>[2x]MQRLGTAVFFLLAFRYSTEQAVGLKEPNAPCTTACGCKSRLLKRLDLYTSKYADGINNERENSEAYSKLVTAALAAVPTMQRKILPLLGAAADILDICRRELATARPLVQAAISKIEEAAGVYNTLHKLERGLG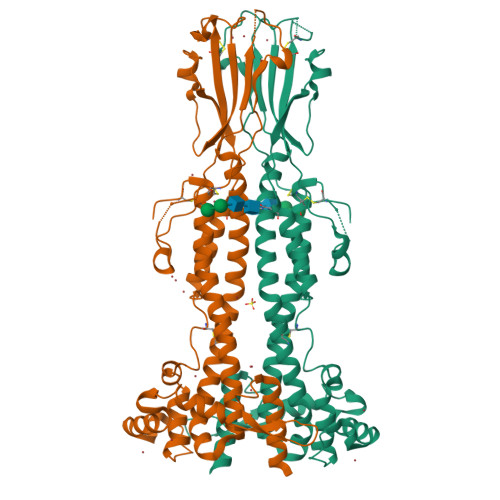EAKIEFGGTDLRLTKTKFRATSLGTIHTADCPNADPGETNVKIGLEHEENEPEPAKLITHGHLDATCASGVGQSSSCHTTAVEANTHLTLGLTFSGSSKDESATWNAATNNKRAIHSNDADFLGSNATVAHEALKAIRSAGASTPCSSLITDFNAVRANPKFKLMVIKALLNKPTAEKESDAPADEVNNAINSAYGREGSEYNTKTWKDIGSTRIPKADPPGEKTDTIDKLSSLPQWGDAIARLLLQEITKQEEQSIKTSSDEATNKECDKHTAKTEGECTKLGCDYDAENKKCKPKSEKETTAAGKKDRAAGETGCAKHGTDKDKCENDKSCKWENNACKDSSILATKKFALSMVSAAFVTLLF>[10x]SFVGLRVVAKWSSNGYFYSGKITRDVGAGKYKLLFDDGYECDVLGKDILLCDP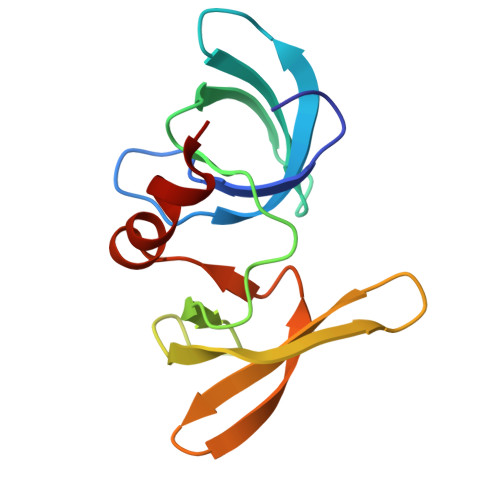IPLDTEVTALSEDEYFSAGVVKGHRKESGELYYSIEKEGQRKWYKRMAVILSLEQGNRLREQYGL> MTDFYTIKDAQADLAIAPLNLTVLLAPYSTTPATTLESPTDGSLAIPPGYKSVGHFEKQAGLTLGNEFDSKDIEAYGEPEPIRTIINKRTTTFDFAMYQNQRNVLELIWTQDFSNIQPSEFGGIVLEAPKVPKNIYYRAILVGMDDRND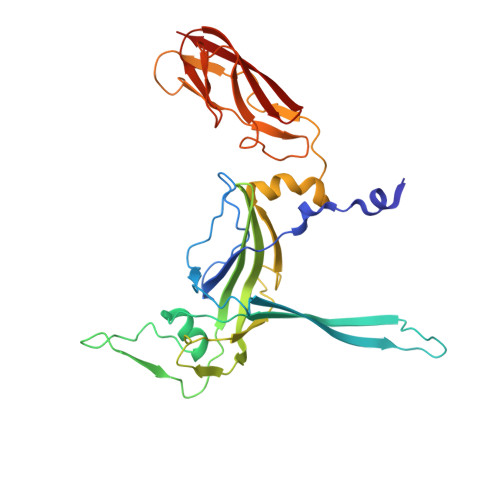RPIWLYWLMPKVKLDKLDNQTLNDDNVIEYKPTLKAFRDDVVGYSVAQGFAGPGWRDLVATAGFGEALTALTITPGSPTVTVATGASHTAQLLVEGDNGINYTPDVVFTSSAPDKASVSAAGLVTGVAAGSATITATKGALTATATVTVTA> MSAGKLPEGWVIAPVSTVTTLIRGVTYKKEQAINYLKDDYLPLIRANNIQNGKFDTTDLVFVPKNLVKESQKISPEDIVIAMSSGSKSVVGKSAHQHLPFECSFGAFCGVLRPEKLIFSGFIAHFTKSSLYRNKISSLSAGANINNIKPASFDLINIPIPPLAEQKIIAEKLDTLLAQVDSTKARFEQIPQILKRFRQAVLGGAVNGKLTEKWRNFEPQHSVFKKLNFESILTELRNGLSSKPNESGVGHPILRISSVRAGHVDQNDIRFLECSESELNRHKLQDGDLLFTRYNGSLEFVGVCGLLKKLQHQNLLYPDKLIRARLTKDALPEYIEIFFSSPSARNAMMNCVKTTSGQKGISGKDIKSQVVLLPPVKEQAEIVRRVEQLFAYADTIEKQVNNALARVNNLTQSILAKAFRGELTAQWRAENPDLISGENSAAALLEKIKAERAASGGKKASRKKS;>MNNNDLVAKLWKLCDNLRDGGVSYQNYVNELASLLFLKMCKETGQEAEYLPEGYRWDDLKSRIGQE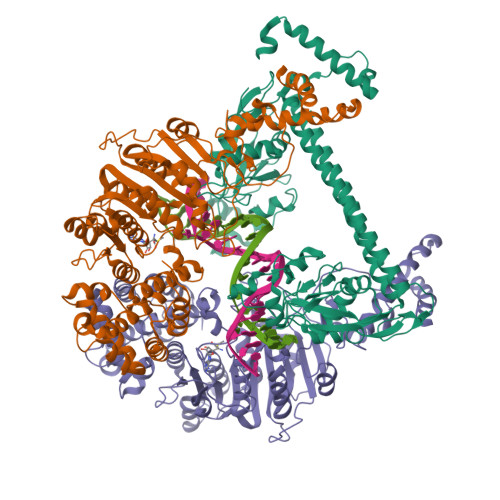QLQFYRKMLVHLGEDDKKLVQAVFHNVSTTITEPKQITALVSNMDSLDWYNGAHGKSRDDFGDMYEGLLQKNANETKSGAGQYFTPRPLIKTIIHLLKPQPREVVQDPAAGTAGFLIEADRYVKSQTNDLDDLDGDTQDFQIHRAFIGLELVPGTRRLALMNCLLHDIEGNLDHGGAIRLGNTLGSDGENLPKAHIVATNPPFGSAAGTNITRTFVHPTSNKQLCFMQHIIETLHPGGRAAVVVPDNVLFEGGKGTDIRRDLMDKCHLHTILRLPTGIFYAQGVKTNVLFFTKGTVANPNQDKNCTDDVWVYDLRTNMPSFGKRTPFTDEHLQPFERVYGEDPHGLSPRTEGEWSFNAEETEVADSEENKNTDQHLATSRWRKFSREWIRTAKSDSLDISWLKDKDSIDADSLPEPDVLAAEAMGELVQALSELDALMRELGASDEADLQRQLLEEAFGGVKE[2x]>MGHHHHHHGEGVQLTAAQELMIQQLVAAQLQCNKRSFSDQPKVTPWPLGADPASGSASQQRFAHFTELAIISVQEIVDFAKQVPGFLQLGREDQIALLKASTIEIMLLETARRYNHETECITFLKDFTYSKDDFHRAGLQVEFINPIFEFSRAMRRLGLDDAEYALLIAINIFSADRP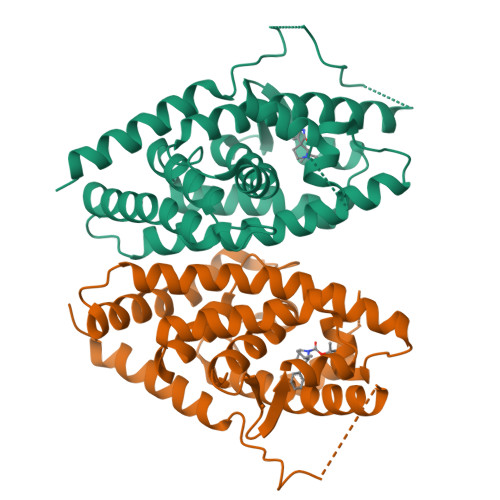NVQEPGRVEALQQPYVEALLSYTRIKRPQDQLRFPRMLMKLVSLRTLSSVHSEQVFALRLQDKKLPPLLSEIWDVHEGSGSGSHKILHRLLQDSSS[4x]> MESYHKPDQQKLQALKDTANRLRISSIQATTAAGSGHPTSCCSAAEIMAVLFFHTMRYKSQDPRNPHNDRFVLSKGHAAPILYAV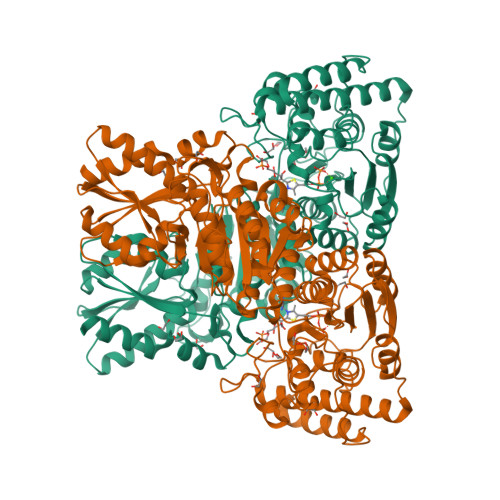WAEAGFLAEAELLNLRKISSDLDGHPVPKQAFTDVATGSLGQGLGAACGMAYTGKYFDKASYRVYCLLGDGELSQGSVWEAMAFASIYKLDNLVAILDINRLGQSDPAPLQHQMDIYQKRCEAFGWHAIIVDGHSVEELCKAFGQAKHQPTAIIAKTFKGRGITGVEDKESWHGKPLPKNMAEQIIQEIYSQIQSKKKILATPPQEDAPSVDIANIRMPSLPSYKVGDKIATRKAYGQALAKLGHASDRIIALDGDTKNSTFSEIFKKEHPDRFIECYIAEQNMVSIAVGCATRNRTVPFCSTFAAFFTRAFDQIRMAAISESNINLCGSHCGVSIGEDGPSQMALEDLAMFRSVPTSTVFYPSDGVATEKAVELAANTKGICFIRTSRPENAIIYNNNEDFQVGQAKVVLKSKDDQVTVIGAGVTLHEALAAAELLKKEKINIRVLDPFTIKPLDRKLILDSARATKGRILTVEDHYYEGGIGEAVSSAVVGEPGITVTHLAVNRVPRSGKPAELLKMFGIDRDAIAQAVRGLITKALVPRGSLEHHHHHH> MGHHHHHHHHHHSSGHIDDDDKHMKNKKDKGLLSGKLTPAQSKNPAKNELYLVEGDSAGGSAKQGRDRKFQAILPLRGKVINTAKAKMADILKNEEINTMIYTIGAGVGADFSIEDANYDKIIIMTDADTDGAHIQTLLLTFFYRYMRPLVEAGHVYIALPPLYKMSKGKGKKEEVAYAWTDGELEELRKQFGKGATLQRYKGLGEMNADQLWETTMNPETRTLIRVTIEDLARAERRVNVLMGDKVEPR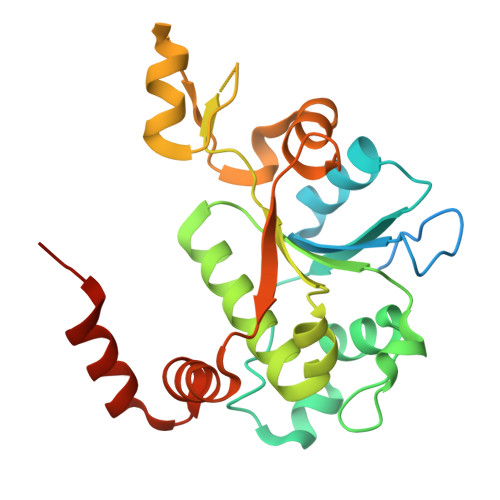RKWIEDNVKFTLEEATVF Several gram-negative bacteria employ type III secretion systems (T3SS) to inject effector proteins into eukaryotic host cells directly from the bacterial cytoplasm. The export gate SctV (YscV in Yersinia) binds substrate:chaperone complexes such as YscX:YscY, which are essential for formation of a functional T3SS. Here, we present structures of the YscX:YscY complex alone and bound to nonameric YscV. YscX binds its chaperone YscY at two distinct sites, resembling the heterotrimeric complex of the T3SS needle subunit with its chaperone and co-chaperone.

The assembly crystallized readily and conditions were identical regardless of which YscX construct (YscXfull-length, YscX32, or YscX50) was used. Diffraction measurement of the ternary complex containing YscVC, YscX32, and His6-YscY gave data to a resolution of 4.1 Å (Supplementray Table 1). Two nonamers are stacked upside-down with their membrane-distal sides interacting in an assembly probably lacking biological significance also described by Kuhlen et al.. Instead, 18 binary complexes were placed manually into helical density present outside of the nonameric YscV rings. Each YscX:YscY complex binds to the SD2-SD4 cleft of an individual YscVC protomer. Minor movements are observed at the binding site between YscY and SD4 as well as helix α3 of YscX and SD4 but these do not seem to affect the export gate globally. Our model also establishes that a highly conserved 46RLYP49 motif of YscX binds within the aforementioned SD2-SD4 cleft. The C-terminal α3 helix—which is the extended helix seen in the YscX:YscY structures—is inserted between two YscVC protomers at the cleft formed between two adjacent SD4 (hereafter referred to as SD4–SD4 cleft). This is the major binding interface between YscV and YscX and involves SD3 and SD4 of YscV. Except for a salt bridge formed between D108 of YscX and R701 of YscVC directly at the entry point for the helix, the interaction is largely hydrophobic with most residues involved being highly conserved. The negative charge of the carboxy-terminus at V122 is presumably neutralized by R551 and R669 of a second YscV molecule. Our structure of the ternary complex YscVC:YscX32:YscY exhibits the same open conformation showing that no major domain rearrangements are necessary to accommodate YscXY.

>MANKGRLGEQEAFAMTVPLLIDVDSSQQEALEAIALNDELVRVRRALYLDLGVPFPGIHLRFNEGMGEGEYLISLQEVPVARGELKAGYLLVRESVSQLELLGIPYEKGEHLLPDQETFWVSVEYEERLEKSQLEFFSHSQVLTWHLSHVLREYAEDFIGIQETRYLLEQMEGGYGELIKEVQRIVPLQRMTEILQRLVGEDISIRNMRSILEAMVEWGQKEKDVVQLTEYIRSSLKRYICYKYANGNNILPAYLFDQEVEEKIRSRVRQTSAGSYLALDPAVTESLLEQVRKTIGDLSQIQSKPVLIVSMDIRRYVRKLIESEYYGLPVLSYQELTQQINIQPLGRVCL[18x];>[18x]GAMGALPPDGHPVEPHLERLYPTAQSKRSLWDFASPGYTFHGLHRAQDYRRELDTLQSLLTTSQSSELQAAAALLKCQQDDDRLLQIILNLLHKV;>MGHHHHHHGNITLTKRQQEFLLLNGWLQLQCGHAERACILLDALLTLNPEHLAGRRCRLVALLNNNQGERAEKEAQWLISHDPLQAGNWLCLSRAQQLNGDLDKARHAYQHYLELKDHNESP[18x]Type I RM enzymes house these activities in a multisubunit complex having ATP-dependent translocation activity that pulls thousands of duplex DNA base pairs through the stationary enzyme, eventually cleaving at random sites distant from the recognition site. Upon identification of an unmethylated specific DNA sequence, two HsdR motor subunits, which bear the endonuclease and ATP-dependent DNA translocation activities in the fully assembled DNA-HsdS-HsdM2-HsdR2 complex, start to translocate the duplex DNA toward the stationary enzyme from both directions, producing two extruded DNA loops flanking the enzyme complex. The X-ray crystal structure of the HsdR subunit with bound ATP from the Type I restriction enzyme of E. coli plasmid R124 revealed four structural and functional domains forming a planar array: one nuclease domain of PD-(E/D)xK type that houses three endonuclease active-site residues and a QxxxY motif common to the RecB-like nucleases; two RecA-like helicase domains of SF2 type that use ATP to translocate duplex DNA without unwinding; and a C-terminal α-helix-rich domain presumed to contact the HsdS-HsdM2 methylase. ATP bound between the two helicase domains was found unexpectedly to also contact Lys220 of the endonuclease domain, suggesting a means by which nuclease and translocation activities might communicate.

The main chain can be traced for residues 217–219 in the Lys220Ala mutant, though with less confidence than in the WT or Lys220Arg structures. In the Lys220Ala and Lys220Glu structures, where the residue 220 sidechain does not form a hydrogen bond with ATP, the helix-like segment is rotated so as to bring the alpha carbon of Asn221 into the position of the alpha carbon of residue 220 in the WT and Lys220Arg structures. In these two structures the Asn221 sidechain points toward ATP and partially fills the space that in the other two structures is occupied by the sidechain of residue 220, but the Asn221 sidechain does not approach the ATP base edge closely enough to hydrogen bond as Lys220 or Arg220 can. A nearby region in 3D space, encompassing residues 181–191 (hereafter 180s loop) is resolved only in the Lys220Ala structure, and there only partially, with the backbone traced confidently through Arg182. Residues 183 to 191 can be traced with less confidence through weak electron density in both monomers of the Lys220Ala asymmetric unit. The resolvability of the 180s loop in the Lys220Ala structure appears to be related to the rotation of the helix-like segment bearing residues 220 and 221. This shift that brings Asn221 into the position of WT Lys220 places Ala220 on the opposite side of the helix-like segment, where its carbonyl group comes within hydrogen-bonding distance (3.2 Å) of the Arg182 guanidino group.

>[2x]MTHQTHTIAESNNFIVLDKYIKAEPTGDSYQSESDLERELIQDLRNQGYEFISVKSQSAMLANVREQLQNLNGVVFNDSEWRRFTEQYLDNPSDGILDKTRKIHIDYICDFIFDDERLENIYLIDKKNLMRNKVQIIQQFEQAGSHANRYDVTILVNGLPLVQIELKKRGVAIREAFNQIHRYSKESFNSENSLFKYLQLFVISNGTDTRYFANTTKRDANSFDFTMNWAKSDNTLIKDLKDFTATCFQKHTLLNVLVNYSVFDSSQTLLVMRPYQIAATERILWKIKSSFTAKNWSKPESGGYIWHTTGSGKTLTSFKAARLATELDFIDKVFFVVDRKDLDYQTMKEYQRFSPDSVNGSENTAGLKRNLDKDDNKIIVTTIQKLNNLMKAESDLPVYNQQVVFIFDECHRSQFGEAQKNLKKKFKRYYQFGFTGTPIFPENALGSETTASVFGRELHSYVITDAIRDEKVLKFKVDYNDVRPQFKSLETETDEKKLSAAENQQAFLHPMRIQEITQYILNNFRQKTHRTFPGSKGFNAMLAVSSVDAAKAYYATFKRLQEEAANKSATYKPLRIATIFSFAANEEQNAIGEISDETFDTSAMDSSAKEFLDAAIREYNSHFKTNFSTDSNGFQNYYRDLAQRVKNQDIDLLIVVGMFLTGFDAPTLNTLFVDKNLRYHGLMQAFSRTNRIYDATKTFGNIVTFRDLERSTIDAITLFGDKNTKNVVLEKSYTEYMEGFTDAATGEAKRGFMTVVSELEQRFPDPTSIESEKEKKDFVKLFGEYLRAENILQNYDEFATLKALQQIDLSDPVAVEKFKAEHYVDDEKFAELQTIRLPADRKIQDYRSAYNDIRDWQRREKEAEKKEKSTTDWDDVVFEVDLLKSQEINLDYILGLIFEHNRQNKGKGEMIEEVKRLIRSSLGNRAKEGLVVDFIQQTNLDDLPDKASIIDAFFTFAQREQQREAEALIKEENLNEDAAKRYIRTSLKREYATENGTELNETLPKLSPLNPQYKTKKQAVFQKIVSFIEKFKGVGGKI> MAPSAVAEPPPIPQRDEPWKRLPPPTVYPVKEARFEKYIPPQLDGRERALAQPPGQVAIVIDNGSHSVRAGWNFEDKPRLAIPPIMSKYRDRKMGKTFSFAGSDCYADTTARSHIRNAFEAGTGIVSNWDVMEHVLDYVFVKLGMNECDGAIDMPIVMTEAVANLPYSRKSMSEIIFECYGAPSLVYGIDSLFSFRHNQGQTGLVVSSSYSATHVIPVYNRKALLSQAIRLNWGGWHMAEYMLKLLKLKYYTGFPGKLNSSQTEHMVRDFCYVSLDYDRELAGYLDWTGLEDRERIVQYPYTEEVVVQKTEEELARIAERKKESGRRLQEQAAKMRLERLMKKEQELEYYKDIQRRMQGESKKEIKRLLDEAELKDEAALERVIRDLERSIKRARQKDLGEPEEEEVPDFSLLDVPDDQLDEAGLRQKRQQRLLKSNWEARQRAKAEKEAEKARLAEEARLDEERRKNDLEGWLEEKRQLRLAKLNQLKERERLKADLGNRKSLASQIRMKNIANLASDNPTGSGSRKRRRGGAGADQDDDFGADDADWGVYRSVAIGANKGDDSDDEEGEEDLEAAIRSLENDLLRYDKTFSYDMTLDAQRDWSKSLLHAFRYGPRPFDPSSQAETHRVHLNVERIRVPEVLFQPAAIAGVDQAGLVEIAGDILCQRLPSLPGIQDAPDAFLR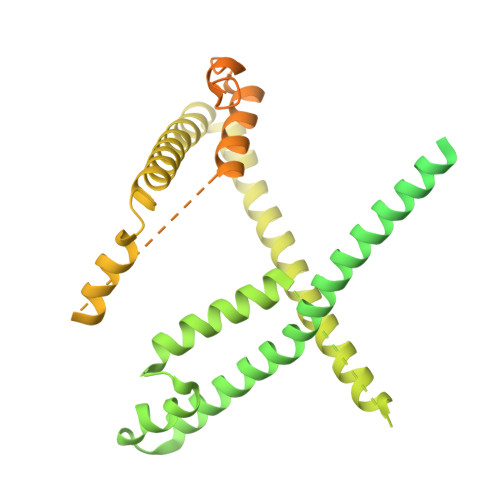DVFLTGGNTLFQNFDERLRQGLMALLPVGAPLRVRRAQDAILDAWRGAAGWACTEEAKAAWITREEYLEKGGEYIKEHDLGNAFA1-(4-{[(2R,3S)-2-{(1R)-1-[3,5-bis(trifluoromethyl)phenyl]ethoxy}-3-(4-fluorophenyl)morpholin-4-yl]methyl}-1H-1,2,3-triazol-5-yl)-N,N-dimethylmethanamine | C26 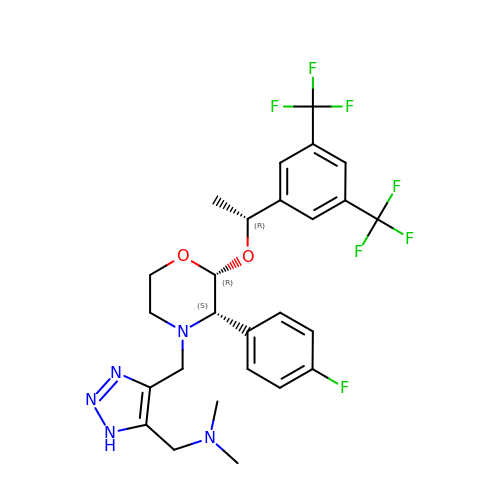H28 F7 N5 O2 | USRYEHHMJIRICK-ZNZBMKLDSA-N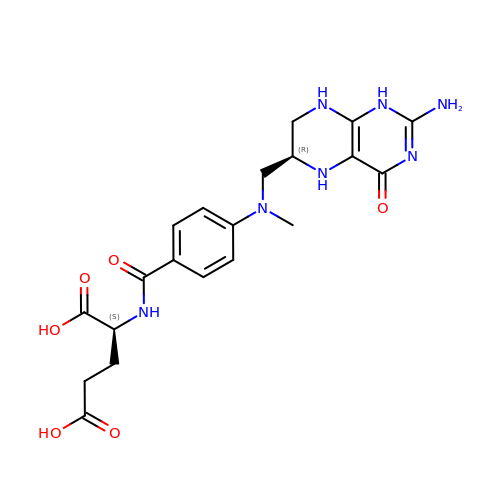(2~{S})-2-[[4-[[(6~{R})-2-azanyl-4-oxidanylidene-5,6,7,8-tetrahydro-1~{H}-pteridin-6-yl]methyl-methyl-amino]phenyl]carbonylamino]pentanedioic acid | C20 H25 N7 O6 | ZHKQAQKGVKBJPP-YPMHNXCESA-N1-(2-fluorobenzene-1-carbonyl)-N-methyl-2,3-dihydro-1H-indole-5-sulfonamide 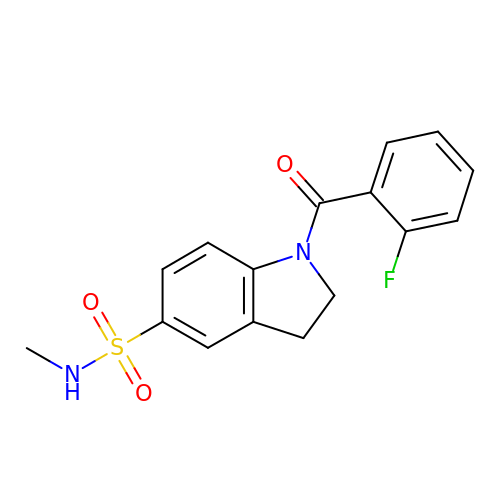| C16 H15 F N2 O3 S | MLAUXXOCJYXBIG-UHFFFAOYSA-N>MKTVVFAYHDMGCLGIEALLAAGYEISAIFTHTDNPGEKAFYGSVARLAAERGIPVYAPDNVNHPLWVERIAQLSPDVIFSFYYRHLIYDEILQLAPAGAFNLHGSLLPKYRGRAPLNWVLVNGETETGVTLHRMVKRADAGAIVAQLRIAIAPDDIAITLHHKLCHAARQLLEQTLPAIKHGNILEIAQRENEATCFGRRTPDDSFLEWHKPASVLHNMVRAVADPWPGAFSYVGNQKFTVWSSRVHPHASKAQPGSVISV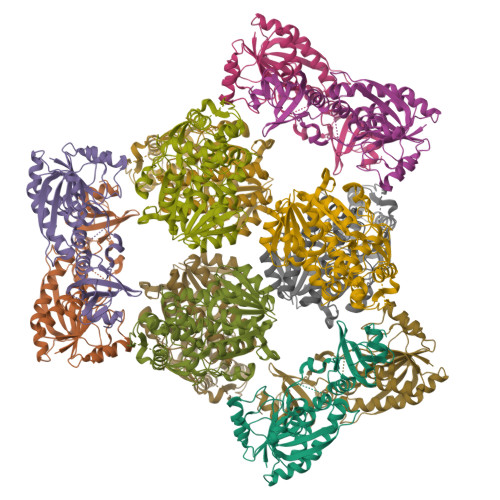APLLIACGDGALEIVTGQAGDGITMQGSQLAQTLGLVQ[6x];>MRVLILGVNGFIGNHLTERLLREDHYEVYGLDIGSDAISRFLNHPHFHFVEGDISIHSEWIEYHVKKCDVVLPLVAIATPIEYTRNPLRVFELDFEENLRIIRYCVKYRKRIIFPSTSEVYGMCSDKYFDEDHSNLIVGPVNKPRWIYSVSKQLLDRVIWAYGEKEGLQFTLFRPFNWMGPRLDNLNAARIGSSRAITQLILNLVEGSPIKLIDGGKQKRCFTDIRDGIEALYRIIENAGNRCDGEIINIGNPENEASIEELGEMLLASFEKHPLRHHFPPFAGFRVVESSSYYGKGYQDVEHRKPSIRNAHRCLDWEPKIDMQETIDETLDFFLRTVDLTDKPS[6x]(R)-2-(3-(2-((4'-Chloro-[1,1'-biphenyl]-2-yl)methyl)-1,2,3,4-tetrahydroisoquinoline-6-carbonyl)-3-(4-methylbenzyl)ureido)-3-((cyclohexylmethyl)sulfonyl)propanoic 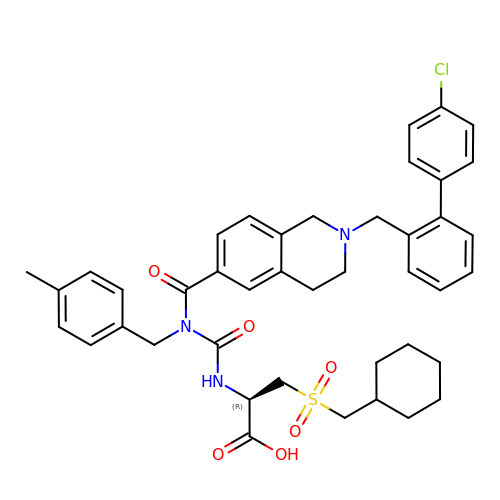acid | C42 H46 Cl N3 O6 S | GZCIVAADWCIZJC-KDXMTYKHSA-N>[2x]MGSIGSMGKPIEGFLVAAIQFPVPIVNSRKDIDHNIESIIRTLHATKAGYPGVELIIFPEYSTQGLNTAKWLSEEF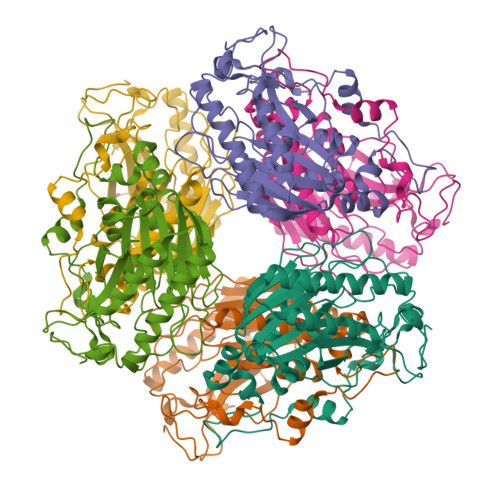LLDVPGKETELYAKACKEAKVYGVFSIMERNPDSNKNPYNTAIIIDPQGEIILKYRKLFPWNPIEPWYPGDLGMPVCEGPGGSKLAVCICHDGMIPELAREAAYKGCNVYIRISGYSTQVNDQWILTNRSNAWHNLMYTVSVNLAGYDNVFYYFGEGQICNFDGTTLVQGHRNPWEIVTGEIYPKMADNARLSWGLENNIYNLGHRGYVAKPGGEHDAGLTYIKDLAAGKYKLPWEDHMKIKDGSIYGYPTTGGRFGK>[2x]MGRIKNKQFAVIGLG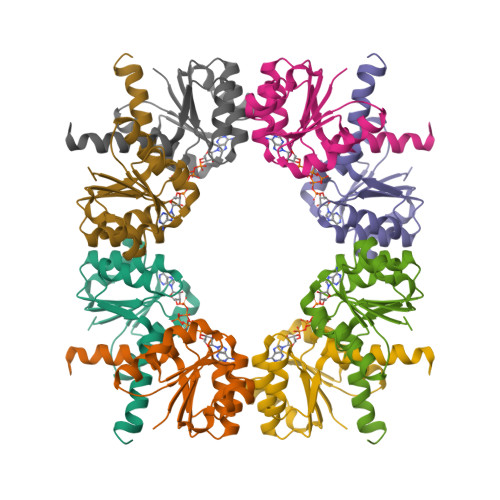RFGGSIVKELHRMGHEVLAVDINEEKVNAYASYATHAVIANATEENELLSLGIRNFEYVIVAIGANIQASTLTTLLLKELDIPNIWVKAQNYYHHKVLEKIGADRIIHPEKDMGVKIAQSLSDENVLNY2-(3-hydroxyphenyl)-N-(pyridin-3-yl)acetamide 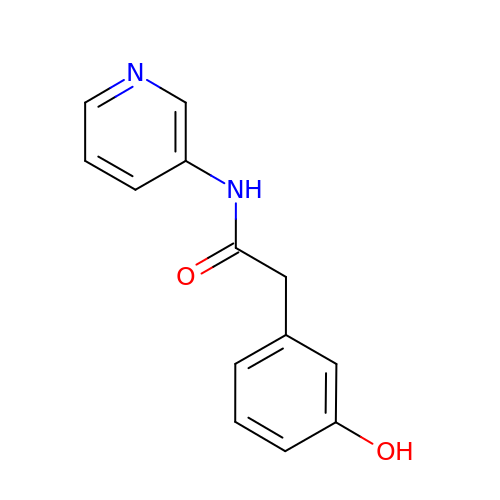| C13 H12 N2 O2 | SVYJPXVRJILISE-UHFFFAOYSA-N> A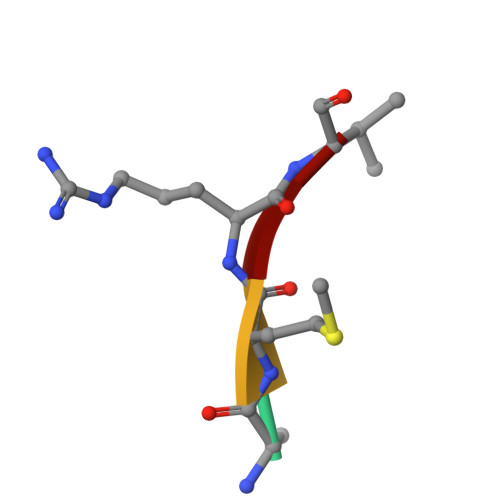MRV>MSQHNEKNPHQHQSPLHDSSEAKPGMDSLAPEDGSHRPAAEPTPPGAQPTAPGSLKAPDTRNEKLNSLEDVRKGSENYALTTNQGVRIADDQNSLRAGSRGPTLLEDFILREKITHFDHERIPERIVHARGSAAHGYFQPYKSLSDITKADFLSDPNKITPVFVRFSTVQGGAGSADTVRDIRGFATKFYTEEGIFDLVGANTPIFFIQDAHKFPDFVHAVKPEPHWAIPQGQSAHDTFWDYVSLQPETLHNVMWAMSDRGIPRSYRTMEGFGIHTFRLINAEGKATFVRFHWKPLAGKASLVWDEAQKLTGRDPDFHRRELWEAIEAGDFPEYELGFQLIPEEDEFKFDFDLLDPTKLIPEELVPVQRVGKMVLNRNPDNFFAENEQAAFHPGHIVPGLDFTNDPLLQGRLFSYTDTQISRLGGPNFHEIPINRPTCPYHNFQRDGMHRMGIDTNPANYEPNSINDNWPRETPPGPKRGGFESYQERVEGNKVRERSPSFGEYYSHPRLFWLSQTPFEQRHIVDGFSFELSKVVRPYIRERVVDQLAHIDLTLAQAVAKNLGIELTDDQLNITPPPDVNGLKKDPSLSLYAIPDGDVKGRVVAILLNDEVRSADLLAILKALKAKGVHAKLLYSRMGEVTADDGTVLPIAATFAGAPSLTVDAVIVPCGNIADIADNGDANYYLMEAYKHLKPIALAGDARKFKATIKIADQGEE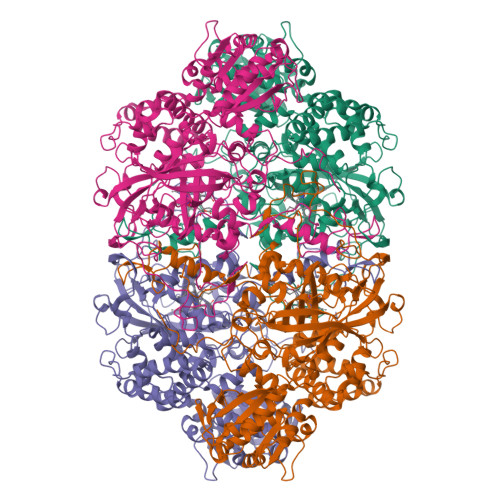GIVEADSADGSFMDELLTLMAAHRVWSRIPKIDKIPA[4x]> MAHFPDTPAFTGFNAPSRIECDIPNLVHEGTIPPELNGAFFRVQPDPQFPPRLGDDISFNGDGMITRFHIHDGQCDIKQRWAKTNKWKLENAAGKALFGSYRNPLTDDESVKGEYRSTANTNAFVFAGKLWAMKEDSPSLTMDPATMETFGFEKFGGKMTGQTFTAHPKVDPLTGNMVAIGYAASGLCTDDVCLYEISPDGELIYEAWFKVPYYCMMHDFGVTKDYLVLHIVPSIGSWDRLEKGLPHFGFDTTLPVYLGIIPRRADLKQEDIRWFKRENCFASHVMNAFQEGTKVHVDVPEAENNMFPFFPDVHGAPFNPQQAMSRLTR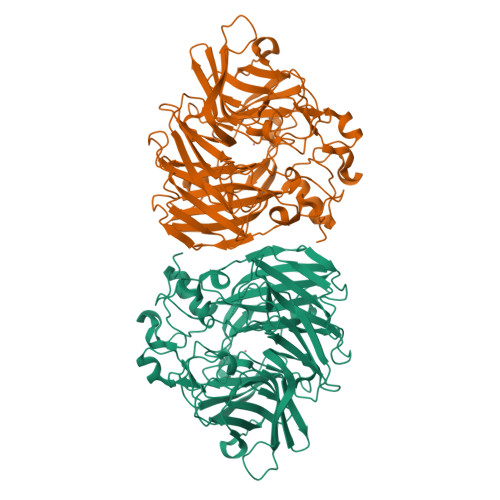WTVDMASNSDEFDSVTRLTETAGEFPRIDDRMTGLPYRYGWMLEMDMKRPVELKGGSAGGFLMNCLFLKDHQTGAEQHWWCGPTSSLQEPAFIPRSKDAPEGDGWIVQVCNRLADHKSDLLIFEALDIEKGPVATVHLPFALRFGLHGNWANAEEIGLAA> SMAEDADMRNELEEMQRRADQLADESLESTRRMLQLVEESKDAGIRTLVMLDEQGEQLERIEEGMDQINKDMKEAEKNLTDLG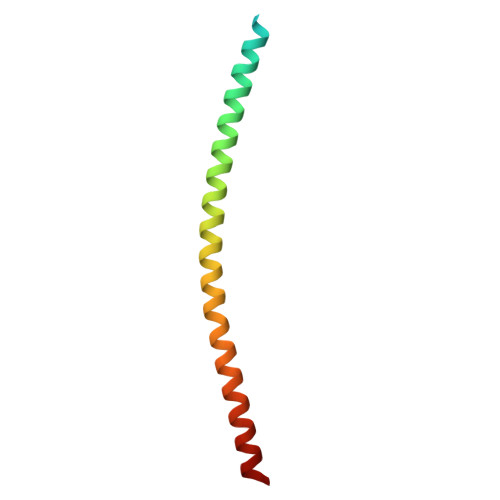K> STVYNINLGIGWASSGVEYAQAYRAQILRRIQQPAKFIFMDMILADNIQHLTENIGFLDEEIIWLYNYFTDIKIAPTTVTLDQVLAQVAGQPERSEKEGKIVRYFYPQDDQFI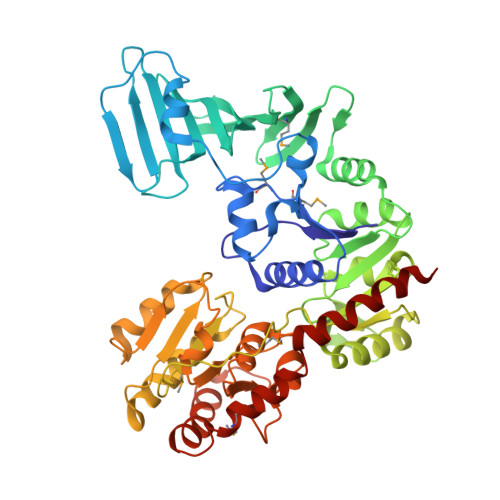TCYLRQEDQDFVEHVEYVSRGRLIRKDYFSYVRYASEYFAPHNDAATLYQRRFYHEDGSVAYDMLIEDGQEKLYRFPDRIFYSKAELVRYFLQCLQLQADDVVILDRETGIGQVVFEESQKAKLGVVVHAEHFSENASSDDYILWNNFYDYQFTNADKVDFFIVATEAQKRILEQQFQHYSDKQPQIATIPVGSLDQLTYPKEPRKPYSMITASRLATEKHIDWLVAATVQAHAQLPELTLDIYGKGSEEDKLRRRIEEAGAQDYIRLKGHADLSQIYAGYELYLTASTSEGFGLTLMEAVGSGLPLIGFDVRYGNQTFIDDGKNGYLLPVSSNHVEDQIIAAFVEKIIALFSQGRQQEMSQHSYQVAENYLTSRVEAAWTQLLKEVRDD>[2x]MLLEAIFHEAKGSYAYPISETQLRVRLRAKKGDVVRCEVLYADRYASPEEELAHALAGKAGSDERFDYFEALLECSTKRVKYVFLLTGPQGEAVYFGETGFSAERSKAGVFQYAYIHRSEVFTTPEWAKEAVIYQIFPERFANGDPSNDPPGTEQWAKDARPRHDSFYGGDLKGVIDRLPYLEELGVTALYFTPIFASPSHHKYDTADYLAIDPQFGDLPTFRRLVDEAHRRGIKIILDAVFNHAGDQFFAFRDVLQKGEQSRYKDWFFIEDFPVSKTSRTNYETFAVQVPAMPKLRTENPEVKEYLFDVARFWMEQGIDGWRLNVANEVDHAFWREFRRLVKSLNPDALIVGEIWHDASGWLMGDQFDSVMNYLFRESVIRFFATGEIHAERFDAELTRARMLYP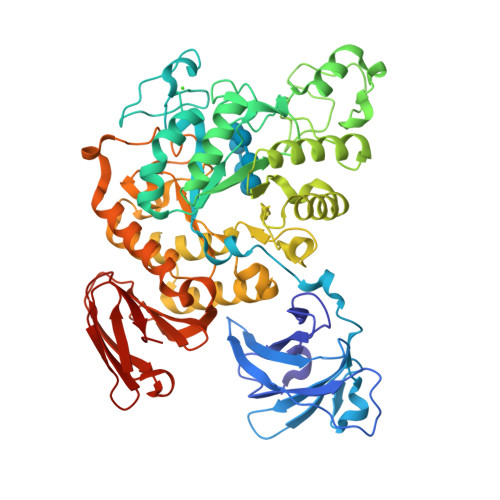EQAAQGLWNLLDSHNTERFLTSCGGNEAKFRLAVLFQMTYLGTPLIYYGDEIGMAGATDPDCRRPMIWEEKEQNRGLFEFYKELIRLRHRLASLTRGNVRSWHADKQANLYAFVRTVQDQHVGVVLNNRGEKQTVLLQVPESGGKTWLDCLTGEEVHGKQGQLKLTLRPYQGMILWNGR> DPMKNTCKLLVVADHRFYRYMGRGEESTTTNYLIELIDRVDDIYRNTAWDNAGFKGYGIQIEQIRILKSPQEVKPGEKHYNMAKSYPNEEKDAWDVKMLLEQFSFDIAEEASKVCLAHLFTYQDFDMGTLGLAYVGSPRANSHGGVCPKAYYSPVGKKNIYLNSGLTSTKNYGKTILTKEADLVTTHELGHNFGAEHDPDGLAECAPNEDQGGKYVMYPIAVSGDHENNKMFSQCSKQSIYKTIESKAQECFQERS;> CTCSPSHPQDAFCNSDIVIRAKVVGKKLVKEGPFGTLVYTIKQMKMYRGFTKMPHVQY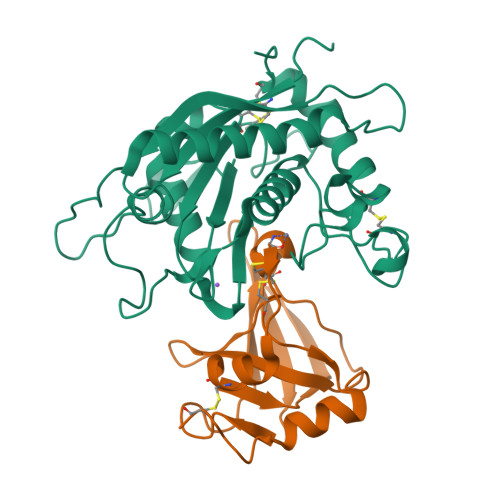IHTEASESLCGLKLEVNKYQYLLTGRVYDGKMYTGLCNFVERWDQLTLSQRKGLNYRYHLGCN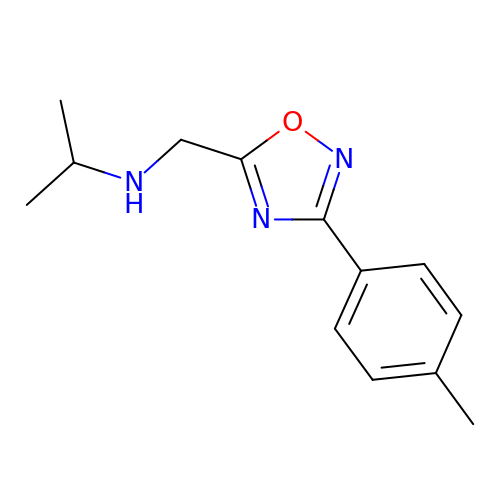~{N}-[[3-(4-methylphenyl)-1,2,4-oxadiazol-5-yl]methyl]propan-2-amine | C13 H17 N3 O | XQOSNFJUNZPHAW-UHFFFAOYSA-N>GSHMRYIDLRSDTVTQPTDAMRQCMLHAEVGDDVYGEDPGVNALEAYGADLLGKEAALFVPSGTMSNLLAVMSHCQRGEGAVLGSAAHIYRYEAQGSAVLGSVALQPVPMQADGSLALADVRAAIAPDDVHFTPTRLVCLENTHNGKVLPLPYLREMRELVDEHGLQLHLDGARLFNAVVASGHTVRELVAPFDSVSICLSKGLGAPVGSLLVGSHAFIARARRLRKMVGGGMRQAGILAQAGLFALQQHVVRLADDHRRARQLAEGLAALPGIRLDLAQVQTNMVFLQLTSGESAPLLAFMKARGILFSGYGELRLVTHLQIHDDDIEEVIDAFTE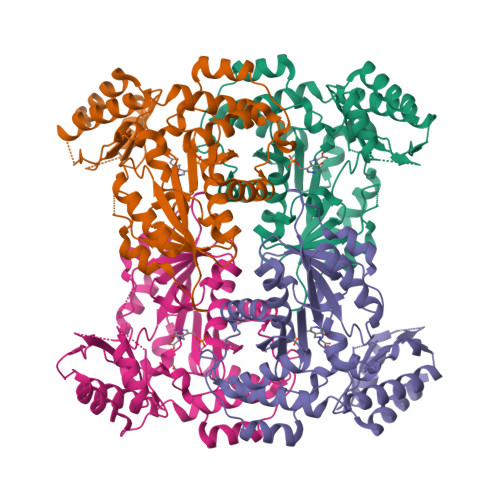YLGA[4x]>[2x]GSVESHPVLEKLKAAHSYNPKEFEWNLKSGRVFIIKSYSE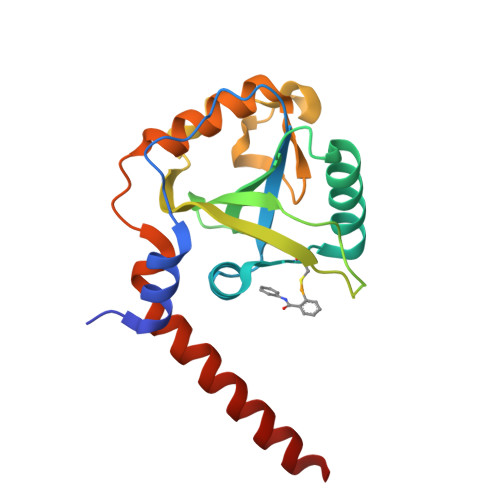DDIHRSIKYSIWCSTEHGNKRLDSAFRCMSSKGPVYLLFSVNGSGHFCGVAEMKSPVDYGTSAGVWSQDKWKGKFDVQWIFVKDVPNNQLRHIRLENNDNKPVTNSRDTQEVPLEKAKQVLKIISSYKHTTSIFDDFAHYEKRQAVVEVVRKERQSRNKQ> HHHHHHADECPTDWKLFDGTCYLFNPSVLHWADAQESCMKEGASLASIHSLEQYTFVKELTTAALTPSWLGGGDCQVSTRWFWMDGTSMD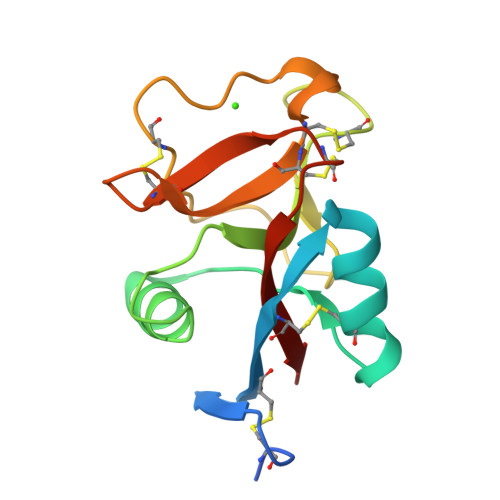FTDWCYAQPDTTLTECCIQMNVGVGKCWDDTPCTHLHSSICAKTST>[72x]MAGGLSQLVAYGAQDVYLTGNPQITFFKTVYRRYTNFAIESIQQTINGSVGFGNKVSTQISRNGDLITDIVVEFVLTKGGNGGTTYYPAEELLQDVELEIGGQRIDKHYNDWFRTYDALFRMNDDRYNYRRMTDWVNNELVGAQKRFYVPLIFFFNQTPGLALPLIALQYHEVKLYFTLASQVQGVNYNGSSAIAGAAQPTMSVWVDYIFLDTQERTRFAQLPHEYLIEQLQFTGSETATPSATTQASQNIRLNFNHPTKYLAWNFNNPTNYGQYTALANIPGACSGAGTAAATVTTPDYGNTGTYNEQLAVLDSAKIQLNGQDRFATRKGSYFNKVQPYQSIGGVTPAGVYLYSFALKPAGRQPSGTCNFSRIDNATLSLTYKTCSIDATSPAAVLGNTETVTANTATLLTALNIYAKNYNVLRIMSGMGGLAYAN;>MPGAISQLVSYGAQDVYLTGNPQITFFKAVYRRYTNFAMESIQQTFDGTTDFGKFPTVTISRNGDLAGPIWIEVNLPSLLGYNITPTPAEGNTSNIAAISTVFKDDYNNYWWTYNPGTTPQYSNLIAAFSNVDYKYYANAVTSTYPPTALSNVVYSWPYMITGNTGTRSTVAIPTANLRYVNGIGLALFNSIELELGGQRIDKHYSEWWDIWTELTETAEKIQGYNTMVGRYDPAVYNAGWNISQAQGGTYYVPLKFCYNRNPGLYMPLVALSYHQMKLNFNINNYLNCVKCNYPVTALTSKNGANPLSITNMKLYTDFVFLDAPERIRMSEIQHEYLVTQLQWQGSEPVTAPGDPNGSTNRKITLNFNHPVRELVFVYQAASNYDVDAVTGNNIFDYEIPANPTATPPYAGGGEVFTEVKLIINGSDRFSGRPGAYFRLVQPYEHHVRVPSKSVYVYSFALEDADSRQPNGSANFTRYDSVQLQLTLNENLASGRVQIYAPNFNILRIAAGMGGLAFAN[8x];> MDPTTRFRGSDVPVHNEDHMVFAKPSEIGLQGRQGFYTNTNVVTNTYNHVYTPPGGHTGGKFTQDIYTTDLLIAAKDEKADKIPLDKRMDGTFSEGTFVQLLSRGPQDVYLTYNPQISLFKRKYKRYTNFAIENFEERFSTVVKFGTRNICQLSKNGDLIGNMCFRVTLPNLGIPGGTWAPTMGYNIFSTIRMRIGDTIVQSHDRVWYDIDDKMFCDSTKIQGLDELIKRNVTLTTDQEWELIIPLKFFCCKRNTGKQQFLPILNMDTNINVYLEFNLLPLNSLVTLPTGSILPDIQSIDASVWVDYIFLDDTEKFRFAQDPCVYLIEQTASMDSLSYATTTSGQTYNKTDVYVDMKELNKPVKYVEIIAYEQGSTSFDYVDIIESATFYLNSDEQFKTRAGEYFSLVQPYQHFKRSDPTSNISTFSFALDAGSFQPNGYLNFAPYVRTRFAFKIQPQTTPHVIRLFAVCLNWVKFESGLVKLLFN;>MSGALNQLVAVGKQDAFITGDNLDNSVWRNVTKKVSNFAMESIENYINVNPGSTTSIVVGRFGDLVRKVTLEITMKKGSTTNPFYPSEQYVKYAHLSIGGQIVYRIDDFPTWTRVHEELFMDPDTRATNQRVNNFRPEDPVGAIRKFYLDIPLFFTDDASKALPLIALQYHEVKLDVLFASPGDIPGIDASYTPTVECYIDYVFLDTPEREWFARNTHMYVIEQLQHYNNVFSVAAVEQTKRLNLPFTMPTRYLIWLLKTGADGVYTTSGYPFENNDSYAAIKSAKLQFNGTDRFSERPGYYFTTVQPQDAFGRSPSAGIYVYSFGLDVTGMTSKGALNFSRMDNATLSITTKAATAATISDVYNQSTTLASAITDFTSIAIYAKSFNVLKIDYGMGGMLFAN[11x];>[4x]MVSGGVVQLISYGAQDVYISGGPKTIFKSYVKKVNNFAIDSVKIPINGMGNGNPSVLIPRNGDLIKSIRLEITLKKGTGQSFYPAEQLISYLALKIGGNIIQKIDDFSNFCRIRNELFMDPDERHTDYRVNNFSSSDVVGSVKYFFLDLPLFFSKDTSVALPLIALQYHDIELDFRFNDVSTIQGVDASYTPTIEMYIDYVYLEQQERIKLVEKPLFYNIEQCNFYRKDITFPALSSTFKLDIPFNNPSRFLVWYFNTDSFGIYNTSGLYFNSNDAAAPLESAVMLLNGTERFKSREGMYFNCVQPQQALGRSPSSGIYMYAFGEDVANATSKGALDMSRVNELSLQLTTKNATAANVYTVYNPQETLASSTSTYKGITLFSTNWNVLQVRSGLGAVMFDS;> MDDIETIEKYGRDETYIFLADSAKRDTAAYPTAAEYEVLFNAQFRNVTKFELLEVNIPRTEYLIDSSENTFAYALNQPTNINTWQQEIEGNIRIATITPGDYNLPQLIDEMNNVLQQTANTYGDSVILQVSPVTNPSEISNKIRITASGPFTLLGSTGTIGNTIGFGDPVNTSVASTTGYYSTVPGYSVNYPNGADYVFLSNQGNIGSEAVNEFVGPLPPGDNVSFTPIYTGQTPSQYFIAPSAGVPTTVSAYFVDQATAPPGGFVVNYSIIKVSDSSTIATGSLISTNDDLVPSVSSPSVVSANFIQGQQYYIQFTPGSSGSSAGNCTALWYSFPNLPPVSGAYAAINGTLVFPGQYFCTDVSAGAYGNELTSPGIVNITGARYIKIRCKELEQLIYRDRVGEPTTAGIGIVNLIGYGFERSRYDFSSIPVKAFHPIGKLQKLTFRLERPNGTLYDTNGVDNTMLCALTFKVVPNNAVDKTFDGPGKYPAAPGYSGDYIQLQQKRWGEEARATYPTHKSTYNRCRPRTT;> MCNTYYKRVKFNLFLYTNSIEMELLAVASIIGYGLFSSQQGRETRPDRNRYAEALGSGQGLDEDYDVKPTDMVRKYRKKAEKRWKKAQVPKESGIITPNMRPSEVMPYFTSGKSMNTNTDYKQRKMELFTGGVLDGHSVSGTYKHKVEAANMFGMTPQGRVTSDGTVGNAPGDTELLKARSVNSHQYNNVLPTEQLRVGPGLGVGPEVAATGGFHQFYRQLPLNINEYKLTQLPGRLVPGGTTTGGKGEIQQIASVNHNPDALVLNYDDRPPEATPNGAILASTQYGKQPRGYAGLRPYEKNYEGIAEADVSALQARYLDQTRGRPRTGDGDTEPIINPNGERDGTGSYVTENMCSMTLESQRGLVNRYITPPGVTGVVQQGGEMRPEFVPETTIREQYEDIYYTGPAGTTVTPTEPMNVVELQPESRHAKRAGQDRAYTPGAGRVNNFAPAAQGAYGLKDHPTYNALQHVVSEPIEQTFLPAAQGDDDRFGTKSNVNNPWGNPASLQIANNQLAANKFNRDVTNTVNLDYDAGQPMKQQNFQPKAWIPNNTDDMKMLPLWKRKQLQAQKNKQQRK;>MAMKTQRKENVLFQNVKPREIPLVDNPFSTYPYKHVITETQPTQAKNQAIWGLVQMGLSGEAAAMYGDVVVQKTTRACRKSEGGFKDVNTELWGTSPYLGRGDGEVYNMPASNQLLRGFESSLRGSRVRTQIDDKSFIPYTWQMIDVPLAAAKTSFIAGLDTRQQLAYGNP[3x];>MFSAFRDTASIGFSDTHQDEKTLRFLKKQISQFIKHLKEYYPNNELTKKLVMKYSDVQLLPYTKGATKDTYTSGLFDHTTGVIKIAPRDGLGNVRDEQSLNKSICHELAHGTRVKYPGESSHSDEWKDAWKTFLKIAADELGWKIEVPCSSVSFYGLTKDDCENCVWDQDPETCPKTAKLA[4x];> MDSRLSAAYAIRAARISMIPGGVDGLVINYAEGGEPAWVQYPLKKQKPLPNNLCYTPTLEDIARKREAVIAKYTKQPLETGTTFTHVLNASHLNEQYTRVKKSALPDKEFPIIETEKYPEPPILWETTIGAPSRLFDRSDGVKYVR;> MILVGIAVLILLAVFAILYYKQKEKFVVVGKFVEPIPSNPGQDFTLLPMDQTYTFADPVPDTATAFDVVLSRFTDKKA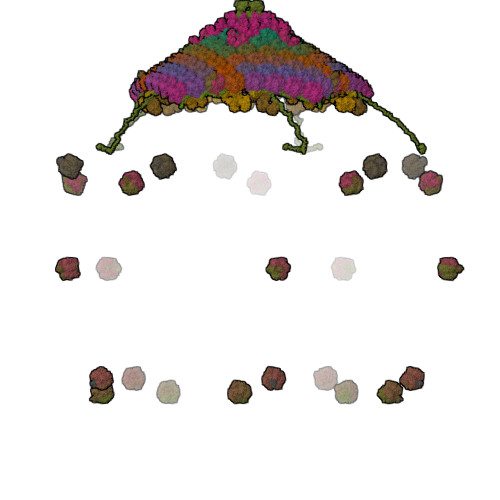PADLLKGATFPEAAPYTDSEVENISKLALSRVKGPDAPVLSFISVEYAAKGVDNKKNTHYDIAFMVYDQVKNFSLKLVLVAVLDAKNKLWIKKFSSFNSFTPKDKGPKGVENIDETPLAEFIPDFVQFSRLYKDNANV;> METIGNFIQNMAFPTENPYKLSGDFGNSTLEPTVTAALRILHESPAPFNTEFFSRKNVDFIQKKLISETKRYTSFDIGPQNEDELIMMMAGIYVQDSTFDGNIKAGLRKLNTLVITECLKQILPGVRAYALYVRDASLPFSGGGEEAFKRPELATLKGSKVLSGFLPLDRNAS;> MKTETLYQDPVWFQDLSVIFKRPSEIIPTRDQSDSERINAMVRLVLYCSFAVALIRQNYLYAILGLAIIAIISLAYALGAKKTKSNEAYGNIRPYSVKRSKKSCSKSSANNPFSNATVGALLDNEARPPACSYDDNDMASTMRKNFNKGLFRNLDDVYEVENSQRQFYTMPVTTAAPDLTAFGQFLYGSKGKTCKEDPSACTPAFATRDG;>[12x]MDMHMIVKVVAILAVLFLVYKLWESMNKPNASPLKIQNPYEKYMNSAEGGEYDAEDDDIYYPETDAEDDDIYTGETDDMYDGEDDDIYVQEGDDIEDAEDEPYDDSADMEQDVPKVQQPMMPLLTPSSQLLPKPSPEAADFAQFAPKNLQAQNFLTATQWIGVNTQGSSLKNANYDLRADPIIPKADVGPWMMSSVDPNIYQKPLFG;>MFLYYKMNEVLNVNNGSSINVIKILKTPGPDIIRPGKTYKKKDVFTPKFFKNGNVMYTCNTFSLNVPVNNSIATIDFAEHVNGAVFKIEYNRVNFIAPSLYPISGLGTAVVFDLQKGEKASQRKITEFGNKDIRIADEISDIAADDHSVLITTKLMSESTPGELSRDVVLNGEIATGRINMNTGFVSDIIHTKKISIIDDGIVDYYVKINVPAKYSHGIVEVVSGTFLNDIMIHLVRNKNKWALMDSKMYIVNNTNGFVIAKNPDTAMGVSLLEWPRGAVVFPPYYNFKKFKNVNKWSISQQIASCVNTSVKIPGGEYSWKIRLFFGPIWQVQESINSVKTVPHGNDYMYLYKEEIVKYKYQRNTKRNFHEYDYDYKF[25x];>[8x]MSGYSNPLNDPIMIRTMIVYGNLSATYFTGNGAALTQQPIASNVPPTLRADAFGNVTSPANVISGNITTIDVISAGNINTRYVFGDGSTLSGISTGNSVVGVQKIDIIGNAVSSTISTGSLRTNVAFTNITANISNISYLSGNTVSNIINASNLIANIVNANVMSGDITLNRIVATDTRTINLFGNVSTNSFTAYGNVTANILTATTLTANSLQIESVSGNSVQKMIVGNLIGNVLTARTATFDTANIPTITSNVGIFTVANIRTITGDVRANVLNVSNIVTRSIGTDVVSNNIIATIGNVQSMIIGNLSANTLSVSNGTFQNFTTTVGLNVTTLSASVSNALVLSFTTGNSSSTTTTNLDAYGNTQFLRISTETSGINILNANSVSVGNLTIVGNVTSTSNNISGQVTSNSSQVQNINTNVIYSGNVFTSRFIAANANIRSLTASIGQVNSLTITSGNLTSLSFVNGNGNGVIATNANISNLNAVSMSGFAFDANVIIGDITANILSSGNLNANVFEANMLTSGNVVSTNGDTGTINANSIVLNVISGGDTRIDRLIANSVTTGDFYTTSTITAGVIDCAQGKISGNSSSNASLISNVISANTASFVNTSVGYGNLVNAVVIGNIIANVVTSGDANAVFLNSNLTTSGSIFGNISNSASIVAEYSNIRTMNVGNINSTTFNAEYLYVGNITVTGVSNTGYLICRNATFSLNSNIQTLITENVTTSNAGSNIFTNVITTGNAFSQNINTINANVLGITSVFSNVITNISNIRTLILLSNVSLGNLTATSANVTSNVSVGNLIGNIVASNAFFNTATIRNLAIFDVTGNILVAQSNASISNLTTERILLSDANIANLSTSNVSSNIAVVTGTCRIDAINSSNITFTNTATVSAAVVNVLGNLTVSNVINVQNLTANVGNIWQAVSNIQSMTTANIFTNTMTIINSFTYSNISSQRLIATNTLTANGVNLFSNIANLTVSGNANVGRWIAASAPATGALCFSSTESANLTTANLFAGNLNTWRAFVGNVIGNVMTTVAGDFGGIRVSVANIDVSGVANVENFTVNGNLFATNVITRDLSANLINFSGSLSNTSSISISGNSLFTSSANAANVGVSINMITQNLFGNRLSSENIQGNVLQASNIAVSQTVNVVGNISIGNLSVSRELFANSITISSGGTIVGNNTTRMITTPTSNSWSVGSLVGNANVSVQFTANTMVVQNIQPNTLVVNINQSTPTSNSGVRAIYIGYIVPVNFNATSSTTVSFSPALPTNCIYMPQLQYYSGGTVLQNNASFSTQIGLGVETITNTSCTIRMSTLDTLPIPSTSFFGLMVTAVQTV;>MSWFDPNWNPFFNRSIIVSGNLVVAGGVIEGNGGGLTNSAFSNPDTIRTDLTGNVTSNGTVRSSLIQTNSIVASGDAYANVWNGNAAFITGISANTTLVGNVRISISGNLTGNFAVSTTTVSNTMTANVLIGTTLTVNNLSATRANVQVLTGNVTGNVRLIANVVNVAAYTVGNLTTSSNVSTTNLNVTSNINGNVRSSTANVQGRLSATTPTTGSIISSSFIANSFTSSGNVQIGDFFGNVRASVGTFDMIASNVFSNVANIIEIRSDIISNIANVGNGTFVFVNASNITTTNITGNITSNVASFSNVDSIFGNVGNLRANTLTVTYANITGTLASGNVAVGNLISADNTSEFANITSFTTNGLVVNGNIIAAIGNGNVFLANVITANSLTLQSSSSTAASNVTTTRWIQSTTSTSNVMTIGNITSGNVISSNAAYFANVISNTITVMSAMTVSGNVSFGNVSFGNVSYGNITANVTTSTGNVSVDNLTSNVVNVVFCNASSVTANTLTSIALTGNTYVYSANTGVLTANVGNVFGTLTVGVANVTSMVSNALFANTAVVSNLSVSNLTVTISSDISNISITGNTSGNVFAANIATIGTLNTANVVANLVASNVMNAWVTSNIRTLITGNANVSTTTSNVITTGGFTITGNITSGLLTSNVIAGNITMYNTSNTTLFTSNTSNIANFFAGNMTAVNTIVSNLEIQGNSVVITQTTPFKVTSVLLANVLFANTIISNTFTTTANVVGNISTDIANIGIANVNFLNTTDFAVNTANIVNYTPTSNINVTGNLTLGNANIVNFYATSANIVGNITANNAVITFLTTPFYKGSGTVSAGFTSIISANALSNVIVFGNLSANIVVSNTLLSNSINVATVFSNVVNIGQVTSTGTTLVNSINFNISNVDVSGNVLVTRDVYTTNISVTTANIANVTFFSNVAIGNLISTRNLTAANLISSSDLFNSGPYTSSQNVTIDTLNFTAGNLGTVAARTTITTPTLFATDVNFTQDALVAGELITQNFYGNITSANIGSRITIGNANVTQTNITGNVVIPRTSNAAGFNSRLLISNNTTVTSNIVANSLISTGNIITNLLQTTGQVSFASLAVEYIDVANLAVRNVVTIGGNLTVSNVANLFSITANTVNMSTVTTNTLSANTITGTSNVLVAGNIIGNCFGNVLVNRGVVTGNVFADTITVPLNAVGVLTGNALIVPNTALHSVAITGSSAFTSNIRTLNTPNAFIWNTSVPSSGLLDARRLRFSQYITSNRIVEMRYFYITNALPQKYDSGGLNARYDLSFGTTLPTSQGQTWHHFLNTLYIGAQYNTNFSINCLIINATTTGLEVIIYNPFGIAASLSSSTPELYFYITSIATSTQ[4x];>MGGIMQLVSTGYQDVFLTGDPTRSLWKRIMARKTNFAIESIETVFDVLYGSTSFINIKKAGDLLKSCVLEITMKRTSTESFYPAEQFIKSLTLLIGDQEVEKIQDFPTWSRVHDELFNDTEMRSANYRMLNFRPDDPPGAIRTFYLDLPLFFTRYLSNSLPLVALQYHEVKLKIDFEPPYNIPGIDSTYMPQVRFYGDYVFLDKPERVYFAQTEHEYIIEQLQTFVTIPNMSNSVNTTMVDLPFTLPSRYIIWVYKTNLHGQYTTSNSTFVTNEGYAPLQSAVIKCNGTDRFSERPGGYFNMVQTTQALGQAPSCGIYMYSFGVNADKQDPEGTLNFSKLDMVTLSYTNKAATAADISQVFDLSTTLENGITKFKNITIFSKNFNVLRIVEGQGGILFSN[3x];>[3x]MGSYFVPPANYFFKDIFASNVGNIANVIFDNGNVIAAGGLGYLIGNGAFITGVTSTAIANIPAVVTADIRGNLIGNYANVNNIIASSGNISNVRFVSGGNVTASYYFGDGSQLTGITATANIPSIVTADIRGNIIGNYANVSNVSATFGNIANVLFNNGNVTAAGGNGFFIGNGSLLTGITATANIPSIVTADIRGNIIGNYANVSNVSATFGNIANVLFNNGNVTAAGGNGYFFGNGALLTGITATANIPSIVTADIRGNIIGNYANVSNVSATFGNIANVLFNNGNVTAAGGNGYFFGNGALLTGITATANIPSIVTADIRGNIIGNYANVSNVSATFGNIANVLFNNGNVTAAGGNGFFIGNGSLLSGITATANIPSIVTADIRGNIIGNYANVSNVTATFGNIANVLFNNGNVTAAGGNGYFFGNGSQLTGVTATLPSIVTADIRGNIIGNYANVSNVIATFGNIANVLFNNGNVTAADGNGYFFGNGSQLTGVTATLPSIVTADIRGNIIGNYANVSNVIATFGNIANVLFNNGNVTAAGGNGYFFGNGALLTGITATANIPSIVTADIRGNIIGNYANVSNVIATFGNIANVLFNNGNVTAADGNGYFFGNGSQLTGVTATLPSIVTADIRGNIIGNYANVSNVIATFGNIANVLFNNGNVTAAGGNGYFFGNGALLTGITATANIPSIVTADIRGNIIGNYANVSNVTATFGNIANVLFNNGNVTAAGGNGYFFGNGSQLTGVTATLPSIVTADIRGNIIGNYANVSNVIATFGNIANVLFNNGNVTAAGGNGYFFGNGALLTGITATANIPSIVTADIRGNIIGNYANVSNVTATFGNIGNVLFNNGNVTAAGGNGYFFGNGTFLNFSTITADIRGNIIGNYANVGNVIAGNVSTTLGNIGNVLFNNGNVTAAGGNGYFFGNGTSLTFSTIRADIRGNIIGNYANVANVIAGNVNSTFGNIAGVTFDAGNVSSPVDILVSGNVSVGSDGLFRGPTNQSNNALILRGIGGTNTVNLFSIGAPSGQMRFSVPASGVAFYNFLYGTNQVASLGPQGFYSLSYDSSVVVGQVVSNSTTYSGTIFKTEANRNSSTAFNHISCTGSNGNVFRVRGDGTTYGVGAFQTSGADYAEMMEWEDKNPTFEDRRGYPVVLSGNGKIRIASLSDDYNNIIGVVSSNPSMLADMAWDQWEGKYLKDKFGMRLSNTIYYLANISNENEFTRVGPMTTPPQGYFIKTSPEYILNPKYNPNVAYVERNDRPEWDPVGFVGKLRVRNGCLVHPSWKPLKVIDDYADVGNAAAQVTEYLIGVTPNYTLSKKVEDLEQTINVLKTQVQMLLGNI;> MGNGPPMERAVSSDDILTYYNTFIFFIYFNFTNENIYIIYTIYMKVQNTIVYIVLLLIVVVIIWNFTRKEGWSDYNAPNDFMKIYYSNIVEDKKLAEKYPFFGTGPFTGLRCRKPNNVGCNTTWVSGQLVELTPKLKEQIECKFGIQYVKT;> MHKITPFLIAAVVAVIVLAVWLFKKDNKKETWFSRDLNYGKANSKIWNATVAKGLKGIANENAEIRKMYPYLGYGDFTGAICKGPNNQGCTYYANYTR;> MWLFFFALAVIYMIYKRDVFKKIAVNLKMNGVSIPFVDKYSKQYPTYTKNALFHVTRFNNAYQKTFEYKNISIDTINNLFSIRDDVLYNISEIKLRLPNDLTQEKEINYMYEKTDQRLMEYITDVKSRFHINIYPGTMSSAFEARNYRASNDIVF;> MQGGLFGTIKLMIMLFSYFAAYQLGKMQERPQSQWPKAKAGQNKYMVGDWAAWKPIYMGVLGVAVLLTLLGPGGVGGGMGGMFGGGGGYGGYY;>MGAFTSFVLMLLFTGIILIATNELTYNRPREIQYRYLPRDLDSFIRTQEMPSAIFSSMWDVDTRRGGDGGPNPPGIRQSN[4x];>[2x]MTTITYDTDLLPPPELKVPSLDQALAPESVKNDDPFLDLSYFPVPKGFDNVGSLELNNLSTAEDVATLQNQLNKLAEEKHKRSTWKGLTFRIAVQDMWEALTGIPTDIYQNSGRVSLKELLTRDDRLRGLGLIFFLVAVVSIFFLAAG;>[3x]MASGWSDFRADPVIVNQDVVVFGNVFVDYLIGNASEMTGAADFVPGNVVNVNIIGNTVSTFVKSDVLMGDTITIDGNITATRLYGDASNMSGLPTLPPNANIDMVGNIVANTNTNKFVSVDTFTGDVTTNVATISNANVGTVTTNTTFFGNVITNVFNIGNLILTSSNVDTLNVTSLVASNVVSSQVDVQATIANSDLNVTRFDATSISAEIFVSSETLAVSNITNLIANIANIQGTTTVTGNLVGNIANVNTLTGNVTGNLFFTNLIIGNITANIFNTTTANVSNLITSNVSASNVSASNVTSTLFTIGNLNTNVATISNLFVTGTTIAGNTTFSSFSVSSLVANISGNNASIPTFTPNVLSTSNITIDGNAVVTGNAGFRTLNVTSLTANVLTTRGDVSNLYTDVINVNTNVFISSANILANNVITVQMNNISNVNITGNAEAFDVSANSVLMSTLSVGGILSLGNVNTNDISFGNIVTGNFFANFANVGNVQGNANVITMYSTTLTSNSAQIGNISGFSIVSNLGNAVSMFVGNLNTGTLVANNSTVGNITYISGNIGNANAQTVRVSGLLSASGVALTFNSITSNVAGNSLTVHGNLRTNSVTTEILTGNVGNLSILNTGNLFANSISVGQSFVISNFANAFIISSQTTNASVITANISGNIRVTNTLEANVVNSDSANIIIKNVSTSGNVSNTFTTGNLTVTNAVFRSGITGNNIEVVGNVNCDGNTTVTTLSYGNLITSVYNTRNIFGNITANTVNITNSNIGNVVTSNINANSLIITNLIPTVDITANVLRASQVNTGWFYGNATCNVLSMSNSVSINTLLSAEVFTSETINANANVSVATINSLGNTVAISRPSFLGNANIRLVISNVITIGNLTANTLVGDSFTATGIVNAINSNSQSDSIATNVTGNIIIRGNLILASSASAQSNASVFNPTNLISLNANSLSSLTATNVSANNVVISNTWQVSNLIVSNISAPNVTANSFQAISMTGRYYRPGISIERAGNLIVSNSLTSTANILQVLTSNTGQVNITNTMFGNISMSNIIVTGVVVTGNLTMGNVIANAVTTSVSTITGNATFGNLTVTDAVIIRGNITANNISTGSYIYGNGAFITGNLTSSGNANISIATRMFGTNSAINVAGTFTGVGNTNTTNATIANLTTNTLLSIGNLSTTGNFTVNSLSVGNLFANGSTIQLSNLANIQVSNLIYSGNVVVSNLSANTLSYVQNIGTSTQLQSGTMNVNNILSAGRFRLSISSTAPVFAGWTMGRVSLSGQSLRTNSGNPRTITFTTPLPAGYSYGIQLSVYSTVFGQTMALFNITVVSLTNTSVQFYIWNNPGGSGDSNTYIGYFAYAY> MAGIAMKLAKDREAAEGLGSHERAIKYLNQDYETLRNECLEAGALFQDPSFPALPSSLGFKELGPYSSKTRGIEWKRPTEICADPQFIIGGATRTDICQGALGDSWLLAAIASLTLNEEILARVVPLDQSFQENYAGIFHFQFWQYGEWVEVVVDDRLPTKDGELLFVHSAEGSE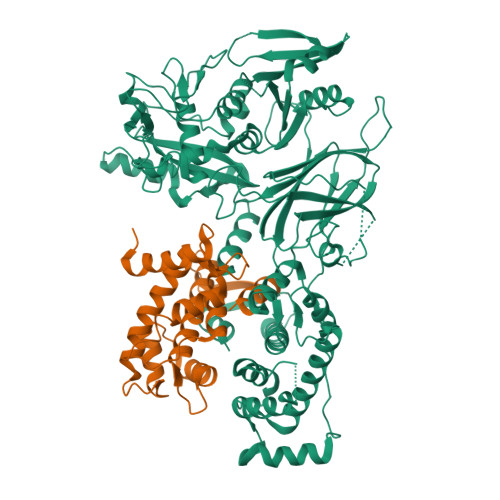FWSALLEKAYAKINGCYEALSGGATTEGFEDFTGGIAEWYELRKPPPNLFKIIQKALEKGSLLGCSIDITSAADSEAVTYQKLVKGHAYSVTGAEEVESSGSLQKLIRIRNPWGQVEWTGKWNDNCPSWNTVDPEVRANLTERQEDGEFWMSFSDFLRHYSRLEICNLTPDTLTCDSYKKWKLTKMDGNWRRGSTAGGCRNYPNTFWMNPQYLIKLEEEDEDDEDGERGCTFLVGLIQKHRRRQRKMGEDMHTIGFGIYEVPEELTGQTNIHLSKNFFLTTRARERSDTFINLREVLNRFKLPPGEYVLVPSTFEPHKNGDFCIRVFSEKKADYQTVDDEIEANIEEIEANEEDIGDGFRRLFAQLAGEDAEISAFELQTILRRVLAKREDIKSDGFSIETCKIMVDMLDEDGSGKLGLKEFYILWTKIQKYQKIYREIDVDRSGTMNSYEMRKALEEAGFKLPCQLHQVIVARFADDELIIDFDNFVRCLVRLEILFKIFKQLDPENTGTIQLDLISWLSFSVL;> MHYSNIEANESEEERQFRKLFVQLAGDDMEVSATELMNILNKVVTRHPDLKTDGFGIDTCRSMVAVMDSDTTGKLGFEEFKYLWNNIKKWQGIYKRFDTDRSGTIGSNELPGAFEAAGFHLNQHIYSMIIRRYSDETGNMDFDNFISCLVRLDAMFRAFRSLDKNGTGQIQVNIQEWLQLTMYS> MKIGIIGAGQLARMLSLAGTPLGLEFHCLGKNGDCAEEVVKTVTDIELTKVNDVV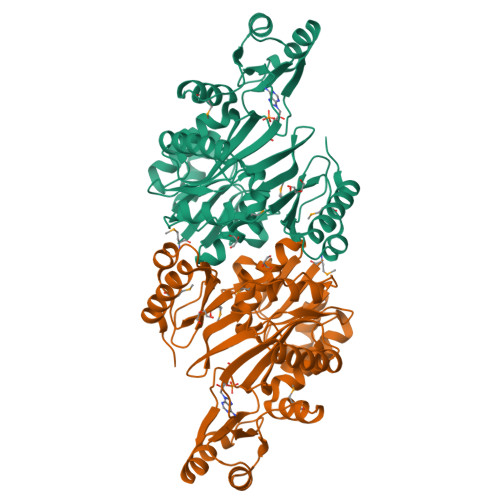AWAKQFDVITFENENISHELIKAINHEVSVYPSAKAIAISQDRLLEKSFMQDHGIATAKFVNIDSLAKLQSAVDDHGLPAILKTRRFGYDGKGQFVIRSQEDITKAWDVLKDAPDGLIYEAFVDFDYEVSQICTADLKGNIAFYPLARNTHKQGIIVESEAPFENVVLAEKAQQIAKILVKEFAYVGTLAIEFFVKGDELIVNEIAPRVHNSGHWSIDGAVTSQFENHVRAIAGLILGDTTSRKTVMLNCIGGMPATKDLAALDRVKIHSYNKEPRKGRKVGHLNLNLNDETDEYQLLQVKKLIALSEEIAGENLYFQ The lipid-enveloped influenza C virus contains a single surface glycoprotein, the haemagglutinin-esterase-fusion (HEF) protein, that mediates receptor binding, receptor destruction, and membrane fusion at the low pH of the endosome. HEF2 is anchored in the viral membrane by a C-terminal transmembrane region and contains an N-terminal hydrophobic fusion peptide. HEF1 forms a receptor-binding domain (R) that recognizes receptors containing 9-O-acetyl sialic acid and an esterase domain (E) that functions as a receptor-destroying 9-O-acetylesterase. In addition, N-terminal and C-terminal segments of HEF1 combine with HEF2 to form the membrane fusion domain (F).

We picked and averaged subtomograms of the envelope from spherical virus particles with a matrix, revealing the 150 Å long trimeric HEF at 9.2 Å resolution. A comparison between the newly obtained map and the crystal structure of the trimeric ectodomain of HEF reveals a dramatic difference in the overall conformation of the molecule. The map and the X-ray model show good agreement in much of the stem region but the maps diverge in the head region where HEF1 domains are splayed out. We applied flexible fitting of the X-ray model to obtain a model for the in situ structure of HEF. Comparison14 of the in situ model with the X-ray model shows points of flexion in both HEF1 (residues 33–34 and 408–409) and HEF2 (residues 65–69 and 99–100). The HEF1 head region in isolation (residues 41 to 371 of HEF1) behaves as a rigid body and itself does not undergo any significant conformational changes in our fitted model compared to the X-ray structure (1.0 Å2 RMSD). The HEF1 head region rotates 20° clockwise (viewed toward the HEF2 stem) and its center of mass is displaced ~7 Å further away from the three-fold axis toward the peripheral density of the nearest neighboring trimer. In the outward position of HEF1 observed in the in situ structure, the HEF2 interhelical loop remains associated with the HEF1 beta-sheet and no longer interposes between long helices allowing the tops of the central helices to associate along the trimer axis (interhelix distance ~12 Å). In the in situ structure, we identify prominent elongated densities on the surface for carbohydrates at N-linked glycosylation sites N12 and N381 of HEF1 and N106 of HEF2 that further validate the fitted model. The in situ “open” conformation of HEF appears to be stabilized by HEF1-HEF1 interactions and the splaying of the membrane distal regions is required to mediate the contacts.

>[3x]EKIKICLQKQVNSSFSLHNGFGGNLYATEEKRMFELVKPKAGASVLNQSTWIGFGDSRTDKSNSAFPRSADVSAKTADKFRFLSGGSLMLSMFGPPGKVDYLYQGCGKHKVFYEGVNWSPHAAINCYRKNWTDIKLNFQKNIYELASQSHCMSLVNALDKTIPLQVTAGTAGNCNNSFLKNPALYTQEVKPSENKCGKENLAFFTLPTQFGTYECKLHLVASCYFIYDSKEVYNKRGCDNYFQVIYDSFGKVVGGLDNRVSPYTGNSGDTPTMQCDMLQLKPGRYSVRSSPRFLLMPERSYCFDMKEKGPVTAVQSIWGKGRESDYAVDQACLSTPGCMLIQKQKPYIGEADDHHGDQEMRELLSGLDYEARCISQSGWVNETSPFTEKYLLPPKFGRCPLAAKEESIPKIPDGLLIPTSGTDTTVTKPKSR;>IFGIDDLIIGVLFVAIVETGIGGYLLGSRKESGGGVTKESAEKGFEKIGNDIQILKSSINIAIEKLNDRISHDEQAIRDLTLEIENARSEALLGELGIIRALLVGNISIGLQESLWELASEITNRAGDLAVEVSPGCWIIDNNICDQSCQNFIFKFNETAPVPTIPPLDTKIDLQ[3x]>[4x]MTAQDITTTLLHPKGDHVLHSHAYPIFQTSTFCFDSTQQGADLFMGKGEGHIYSRLGNPTVEQFEEMVCSIEGAAGSAAFGSGMGAISSSTLAFLQKGDHLIAGDTLYGCTVSLFTHWLPRFGIEVDLIDTSDVEKVKAAWKPNTKMVYLESPANPTCKVSDIKGIAVVCHERGARLVVDATFTSPCFLKPLELGADIALHSVSKYINGHGDV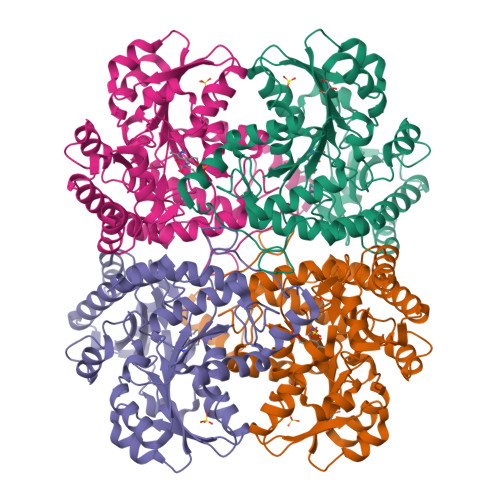IGGVSSAKTAEDIATIKFYRKDAGSLMAPMDAFLCARGMKTLPIRMQIHMENGLKVAKFLEQHEKIVKVNHPGLESFPGHDIAKKQMTGYGSTFLFEMKSFEAAKKLMEHLKVCTLAVSLGCVDTLIEHPASMTHAAVPENIMRKQGITPELVRISVGIENVDDIIADLKQALELW>[3x]GCGTAEVTTSNAPSEEVTAVTTEVQGETEEKKKVLTTFTVLADMVQNVAGDKLVVESITRIGAEIHGYEPTPSDIVKAQDADLILYNGMNLERWFEQFLGNVKDVPSVVLTEGIEPIPIADGPYTDKPNPHAWMSPRNALVYVENIRQAFVELDPDNAKYYNANAAVYSEQLKAIDRQLGADLEQVPANQRFLVSCEGAFSYLARDYGMEEIYMWPINAEQQ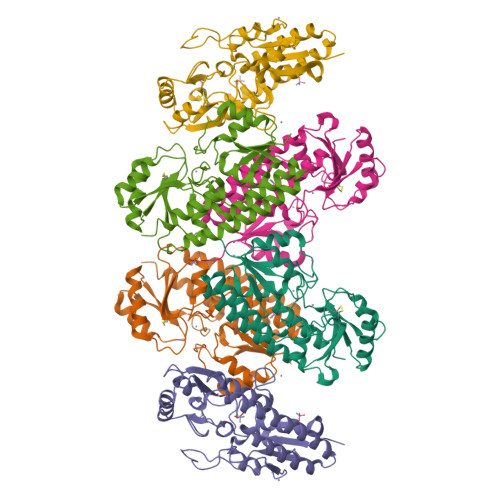FTPKQVQTVIEEVKTNNVPTIFCESTVSDKGQKQVAQATGARFGGNLYVDSLSTEEGPVPTFLDLLEYDARVITNGLLAGTNAQQ>[2x]SSS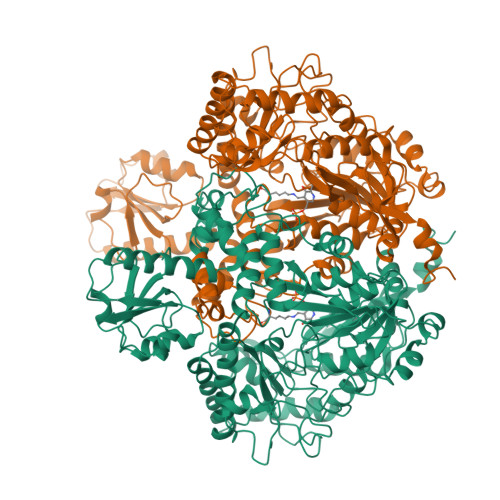LKIASTQEARQYFDTDRVVVDAVGSDFTDVGAVIAMDYETDVIDAADATKFGIPVFAVTKDAQAISADELKKIFHIIDLENKFDATVNAREIETAVNNYEDSILPPFFKSLKEYVSRGLIQFDCPGHQGGQYYRKHPAGREFYDFFGETVFRADLCNADVALGDLLIHEGPAVAAEKHAARVYNADKTYFVLGGSSNANNTVTSALVSNGDLVLFDRNNHKSVYNSALAMAGGRPVYLQTNRNPYGFIGGIYDSDFDEKKIRELAAKVDPERAKWKRPFRLAVIQLGTYDGTIYNAHEVVKRIGHLCDYIEFDSAWVGYEQFIPMMRNSSPLLIDDLGPEDPGIIVVQSVHKQQAGFSQTSQIHKKDSHIKGQLRYCDHKHFNNSFNLFMSTSPFYPMYAALDVNAAMQEGEAGRKLWHDLLITTIEARKKLIKAGSMFRPFVPPVVNGKKWEDGDTEDMANNIDYWRFEKGAKWHAYEGYGDNQYYVDPNKFMLTTPGINPETGDYEDFGVPATIVANYLRDHGIIPEKSDLNSILFLMTPAETPAKMNNLITQLLQLQRLIEEDAPLKQVLPSIYAANEERYNGYTIRELCQELHDFYKNNNTFTYQKRLFLREFFPEQGMLPYEARQEFIRNHNKLVPLNKIEGEIALEGALPYPPGVFCVAPGEKWSETAVKYFTILQDGINNFPGFAPEIQGVYFKQEGDKVVAYGEVYDAEVAKNDDRYNN> MAAPAAEAPLSHVQQALAELAKPKDDPTRKHVCVQVAPAVRVAIAETLGLAPGATTPKQLAEGLRRLGFDEVFDTLFGADLTIMEAGSELLHRLTEHLEAHPHSDEPLPMFTSCCPGWIAMLEKSYPDLIPYVSSCKSPQMMLAAMVKSYLAEKKGIAPKDMVMVSIMPCTRKQSEADRDWFCVDADPTLRQLDHVITTVELGNIFKERGINLAELPEGEWDNPMGVGSGAGVLFGTTGGVMEAALRTAYELFTGTPLPRLSLSEVRGMDGIKETNITMVPAPGSKFEELLKHRAAARAEAAAHGTPGPLAWDGGAGFTSEDGRGGITLRVAVANGLGNAKKLITKMQAGEAKYDFVEIMACPAGCVGGGGQPRSTDKAITQKRQAALYNLDEKSTLRRSHENPSIRELYDTYLGEPLGHKAHELLHTHYVAGGVEEKDEKKSAWSHPQFEK

[FeFe]-hydrogenases represent one of natures’ most effective classes of redox enzymes catalyzing the reversible reduction of protons to dihydrogen (H2) at turnover frequencies of up to 9000 s-11–3. With their low catalytic over-potential, [FeFe]-hydrogenases represent excellent models for a regenerative and likewise economically feasible H2 production. Their active center (“H-cluster”) can be structured into a standard [4Fe-4S]-cluster ([4Fe]H) and a diiron site ([2Fe]H). Theoretical studies suggest that the most probable PT pathway comprises of strictly conserved residues E282, S319, E279, and C299 (from surface to H-cluster, numbering corresponds to CpI), including two protein-bound water molecules (Wat826, Wat1120 4XDC19, chain B) located between E279 and C29915,16,20. In this study, site-directed mutagenesis (SDM) is used to investigate the PT pathway of two [FeFe]-hydrogenases, namely CpI and HydA1, which represent the largest (M3) and smallest (M1) type of monomeric [FeFe]-hydrogenases, respectively.

Crystallization of HydA1 exclusively succeeded for apo-protein, which carries the [4Fe]H-cluster but lacks the [2Fe]H-site. Variants of HydA1 apo-protein were crystallized in space group P32 2 1, with a single chain in the asymmetric unit. However, comparisons of crystal structures of CpI apo- and holo-protein with apo-HydA1 demonstrated that a lack of cofactor does not affect the configuration of the putative PT pathway. For the corresponding alanine variant of both, HydA1 and CpI, shifts of the conserved water molecule in the putative PT pathway can be observed. While glutamine occupies the entire space of the native carboxyl group and thus clearly interrupts the putative PT pathway, an exchange to alanine may support additional H2O molecules to bridge the gap.2-cyano-3-[4-(dimethylamino)phenyl]-~{N}-[(2~{R},3~{R},4~{S},5~{S},6~{R})-6-(hydroxymethyl)-3,4,5-tris(oxidanyl)oxan-2-yl]propanamide | C18 H23 N3 O6 | 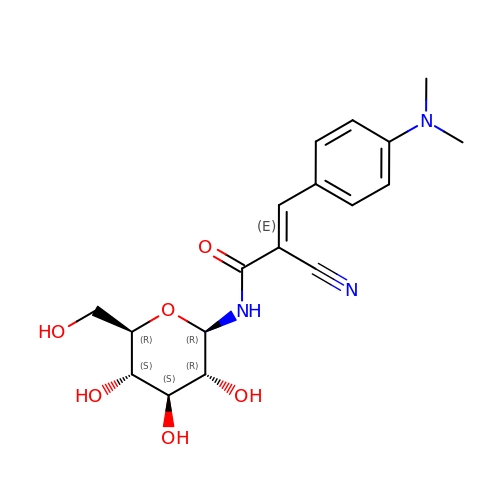QKTHDRCOMWPULY-NBXQZZMVSA-N>[4x]AEPQPPSGGLTDEAALSCCSDADPSTKDFLLQETMLRVKDPKKSLDFYTRVLGMTLIQKCDFPIMKFSLYFLAYEDKNDIPKEKDEKIAWALSRKATLELTHNWGTEDDETQSYHNGN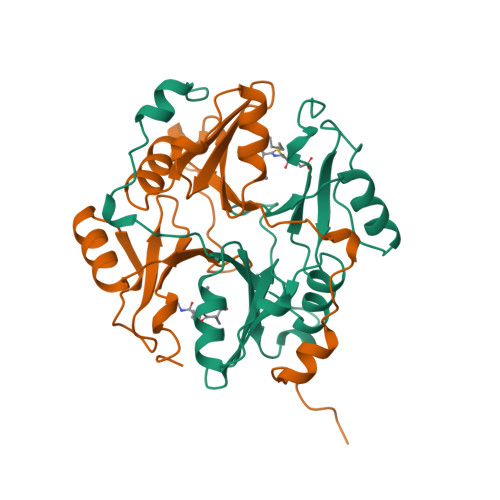SDPRGFGHIGIAVPDVYSACKRFEELGVKFVKKPDDGKMKGLAFIQDPDGYWIQILNPNKMATLM>KHSLPDLPYDYGALEPHINAQIMQLHHSKQHAAYVNNLNVTEEKYQEALAKGDVTAQIALQPALKFNGGGHINHSIFWTNLSPNGGGEPKGELLEAIKRDFGSFDKFKEKLTAASVGVQGSGWGWLGFNKERGHLQIAA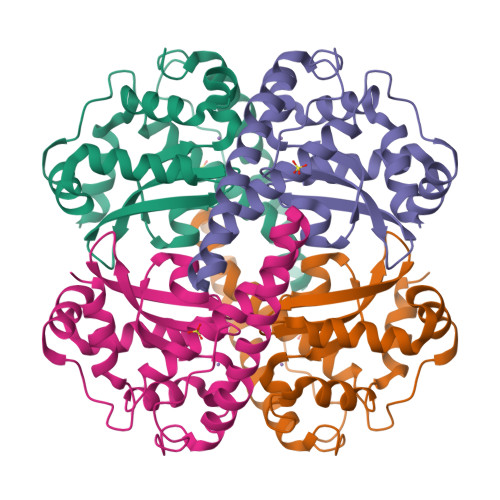CPNQDPLQGTTGLIPLLGIDVWEHAYYLQYKNVRPDYLKAIWNVINWENVTERYMACKK[2x]> KRQWALEDFEIGRPLGKGKFGNVYLAREKQSKFILALKVLFKAQLEKAGVEHQLRREVEIQSHLRHPNILRLYGYFHDATRVYLILEYAPLGTVYRELQKLSKFDEQRTATYITELANALSYCHSKRVIHRDIKPENLLLGSAGELKIADFGWSVHAPSSRRTTLCGTLDYLPPEMIEGRMHDEKVDLWSLGVLCYEFLVGKPPFEANT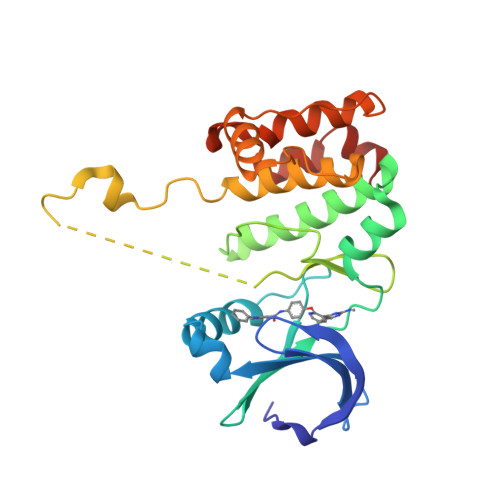YQETYKRISRVEFTFPDFVTEGARDLISRLLKHNPSQRPMLREVLEHPWITANSSKPS> KDNIRHGVCWIYYPDGGSLVGEVNEDGEMTGEKIAYVYPDERTALYGKFIDGEMIEGKLATLMSTEEGRPHFELMPGNSVYHFDKSTSSCISTNALLPDPYESERVYVAESLISSAGEGLFSKVAVGPNTVMSFYNGVRITHQEVDSRDWALNGNTLSLDEETVIDVPEPYNHVSKYCASLGHK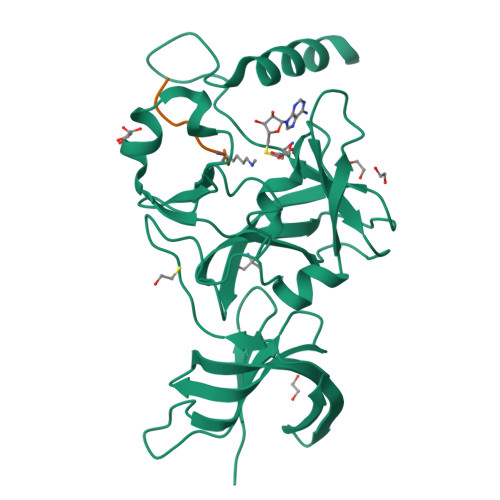ANHSFTPNCIYDMFVHPRFGPIKCIRTLRAVEADEELTVAYGYDHSPPGKSGPEAPEWYQVELKAFQATQQK;> TPRRSKSA>GPGGSGGMKPQIRNMVEPMDPRTFVSNFNNRPILSGLDTVWLCCEVKTKDPSGPPLDAKIFQGKVYPKAKYHPEMRFLRWFHKWRQLHHDQEYKVTWYVSWSPCTRCANSVATFLAKDPKVTLTIFVARLYYFWDPDYQQALRILAEAGATMKIMNYNEFQDCWNKFVDGRGKPFKPWNNLPKHYTLLQATLGELLRHLMDPGTFTSNFNNKPWVSGQHETYLCYKVERLHNDTWVPLNQHRGFLRNQAPNIHGFPKGRHAALCFLDLIPFWKLDGQQYRVTCFTSWSPCFSCAQEMAKFISNNEHVSLCIFAARIYDDQGRYQEGLRTLHRDGAKIAMMNYSEFEYCWDTFVDRQGRPFQPWDGLDEHSQALSGRLRAILQNQGN[2x]

Human APOBEC3G (hA3G) is a member of apolipoprotein B mRNA editing enzyme catalytic polypeptide like (APOBEC) family, and is one of the most effective antiviral host restriction factors against exogenous retroviral pathogens such as human immunodeficiency virus type 1 (HIV-1) and endogenous retroviral derived remnants on the human genome. hA3G is a DNA/RNA cytidine deaminase converting 3′ target cytidine (C) in 5′-CC-3′ or 5′-CCC-3′ motif to uridine (U) within single-stranded DNA (ssDNA)9–15 or single-stranded RNA (ssRNA). hA3G has two cytidine deaminase domains in tandem, the N-terminal CD1 (or NTD) and C-terminal CD2 (or CTD). The ability to bind nucleic acids and form oligomerization is attributed mainly to CD1/NTD (referred to as CD1 hereafter), while deaminase activity is performed by CD2/CTD (referred to as CD2 hereafter). In this study, we describe four structures of a soluble primate rA3G variant from rhesus macaque, rA3GR8/E259A, in complex with AA and GA dinucleotide-containing RNA molecules in the form of ssRNA and dsRNA with 5′- or 3′-overhangs.

Additionally, RNA1-AA was modified to 5′ U1U2A3A4-dsRNA8-C13C14U15U16U17U18 with 5′ and 3′ overhangs on both strands (designated as RNA1-AAxtal, with dsRNA8 5′-CGCUGCGG-3′/5′-CCGCAGCG-3′). Complexes with RNA1-AAxtal and RNA2-AAxtal were determined as two different types of dimers with two rA3G molecules binding to one RNA molecule at 2.90 and 3.10 Å, respectively. In both cases, the electron density maps of RNA were of sufficient quality to allow de novo building of a complete dsRNA8 plus three nucleotides (3-nt) on each AA dinucleotide-containing overhang (5′-U2A3A4-dsRNA8-3′ and 5′-dsRNA8-A9A10U11-3′). In both dimer models, there are no direct contacts between the two rA3GR8/E259A monomers, which is reminiscent of A3H-dsRNA complexes showing RNA-assisted dimer formation. Averaged RNA surface area buried with one rA3GR8/E259A is ~820 Å2 in RNA1-AAxtal and ~841 Å2 in RNA2-AAxtal. With two rA3GR8/E259A monomers contacting one RNA, approximately 1640 to 1680 Å2 of the RNA surface area centered around the AA dinucleotides was buried in a rA3G-RNA dimer, which accounts for roughly 28% of the total RNA surface area, leaving most of the dsRNA surface exposed. In the 5′-overhang dsRNA co-crystal structure, dsRNA8 has little contact with rA3G, resulting in a relatively weaker electron density for part of the dsRNA. A C-G base pair (C5-G12) 3′ to the bound AA core (5′-A3A4-3′) is hovering over the surface of CD1-loop 3 (58VYP60). The side chain of the loop 3 residue Y59 shows no clear electron density at 1 sigma contour level, suggesting it doesn’t make strong contact with the RNA. When in complex with 5′- or 3′-overhang dsRNA containing unpaired AA dinucleotide, RNA-mediated rA3G dimers are formed.> MHHHHHHMKHNQLPLVIEFTEQTAPKIFGGEIKTHIL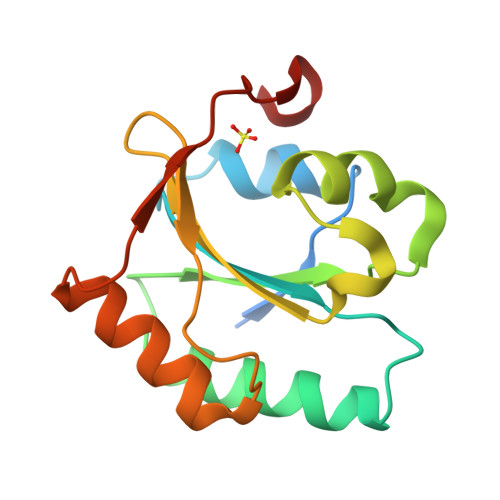LFLPKSVSDYDGKLSNFKTAAESFKGKILFAFIDSDHTDNQRILEFFGLKKEECPAVRLITLEEEMTKYKPESEELTAERITEFCHRFLEGKIKPHLMSQELPEDWDKQP> MSVPAGSVSCLANALLNLRSSTDYNADHGVKNSILNFSNSKDASRFDGSESWSSSVLDKNQFIVA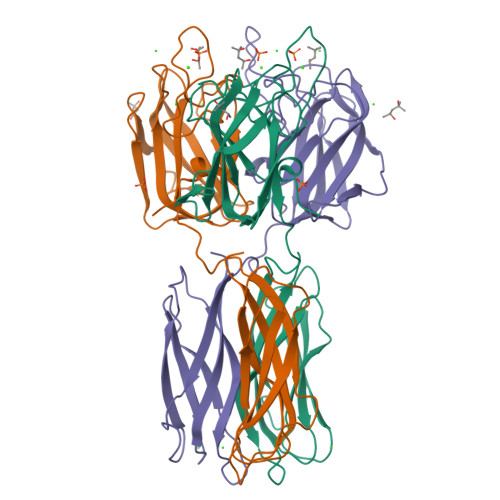GSDSVKHFVAISTQGRGDHDQWVTSYKLRYTLDNVNWVEYNNGEIINANKDRNSIVTINFNPPIKARSIAIHPQTYNNHISLRWELYALPVKSYSNPSVQVGEVSIGDRSLNSGTGSRTIVRHVKFPVEFLSVPIVSIGCKKVDAHTDNGQMRWEGKSENITTKGFDLTFITWGNNAVYDLTFDYVAVEFNN(4~{Z})-4-(1,3-benzothiazol-6-ylmethylidene)-2-[[(2~{R})-1-methoxy-4-methyl-pentan-2-yl]amino]-1~{H}-imidazol-5-one | C18 H22 N4 O2 S | 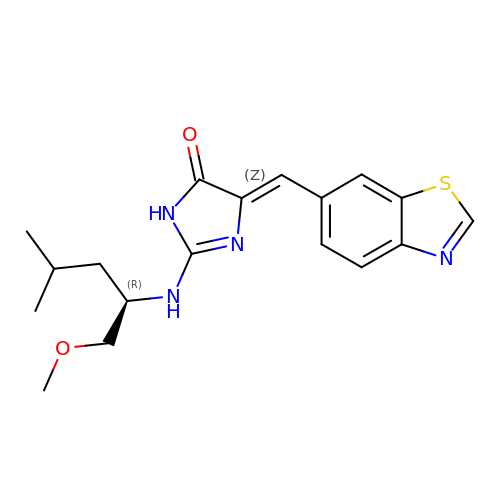CHQYAWLKOUOTQO-QVYJARAXSA-N> MPVNIKNFNYNDPINNDDIIMMEPFNDPGPGTYYKAFRIIDRIWIVPERFTYGFQPDQFNASTGVFSKDVYEYYDPTYLKTDAEKDKFLKTMIKLFNRINSKPSGQRLLDMIVDAIPYLGNASTPPDKFAANVANVSINKKIIQPGAEDQIKGLMTNLIIFGPGPVLSDNFTDSMIMNGHSPISEGFGARMMIRFCPSCLNVFNNVQENKDTSIFSRRAYFADPALTLMHELIHVLHGLYGIKISNLPITPNTKEFFMQHSDPVQAEELYTFGGHDPSVISPSTDMNIYNKALQNFQDIANRLNIVSSAQGSGIDI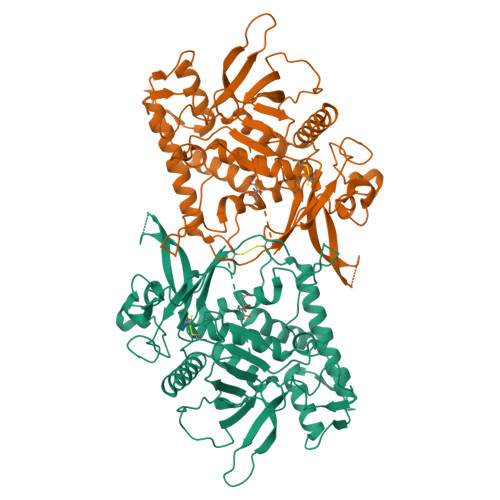SLYKQIYKNKYDFVEDPNGKYSVDKDKFDKLYKALMFGFTETNLAGEYGIKTRYSYFSEYLPPIKTEKLLDNTIYTQNEGFNIASKNLKTEFNGQNKAVNKEAYEEISLEHLVIYRIAMCKPVMYKNAPPTPGHHHHHH>[9x]MNEGRIFLYVSPEVILPIMFLIL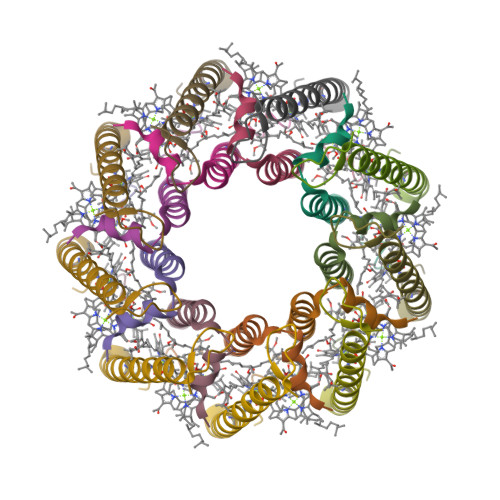VLTSLTVHFAILINTTWFGDFFQGSAGEFAAAPAAADANAAPWE;>MAGDDTKVYPTGLTEAQALEINDGLKWGTRIYFGIAVAAHILAFILTPWLK[9x]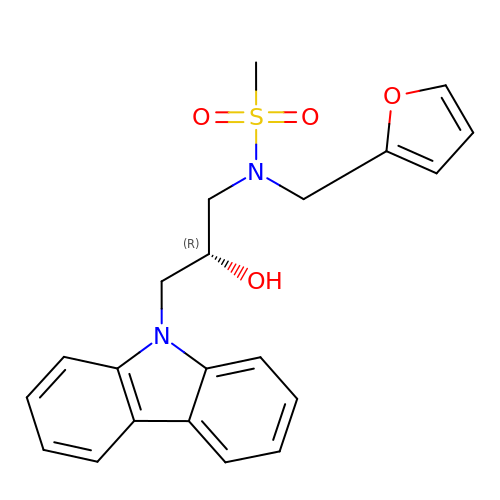N-[(2R)-3-carbazol-9-yl-2-oxidanyl-propyl]-N-(furan-2-ylmethyl)methanesulfonamide | C21 H22 N2 O4 S | OQAFDLPAPSSOHY-INIZCTEOSA-N N-[(R)-(2-amino-5-chloro-3-fluoropyridin-4-yl){7-[4-(2-hydroxypropan-2-yl)pyridin-2-yl]-1-benzothiophen-2-yl}methyl]cyclopropanesulfonamide | C25 H24 Cl F N4 O3 S2 | 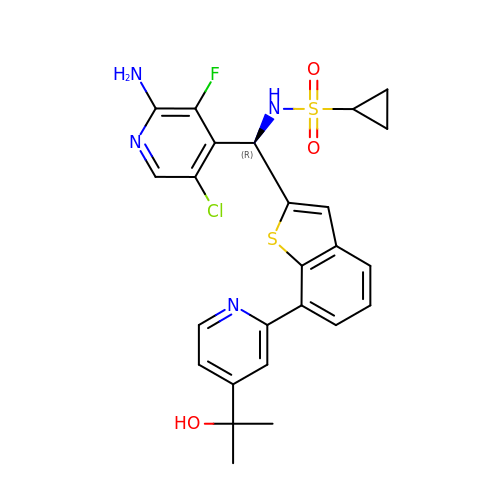FBKAQPKUCXZNGQ-QFIPXVFZSA-N> TSWRSEATFQFT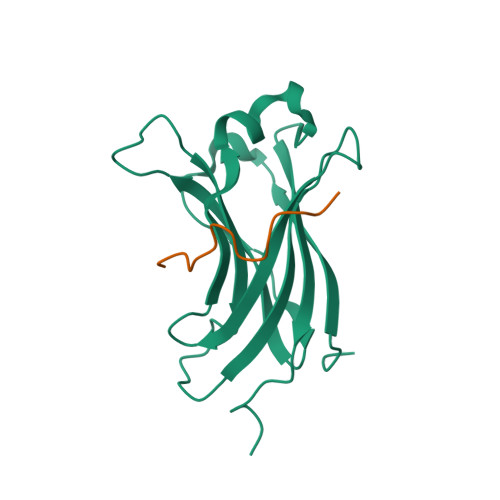VERFSRLSESVLSPPCFVRNLPWKIMVMPRFYPDRPHQKSVGFFLQCNAESDSTSWSCHAQAVLKIINYRDDEKSFSRRISHLFFHKENDWGFSNFMAWSEVTDPEKGFIDDDKVTFEVFVQADAPHGVAW;> SVWIPVNEGASTSGM> GLGDELEEVIVEKTKQTVASISSGPKHTQKVPILTANETGATMPVLPSDSIETRTTYMHFNGSETDVECFLGRAACVHVTEIQNKDAT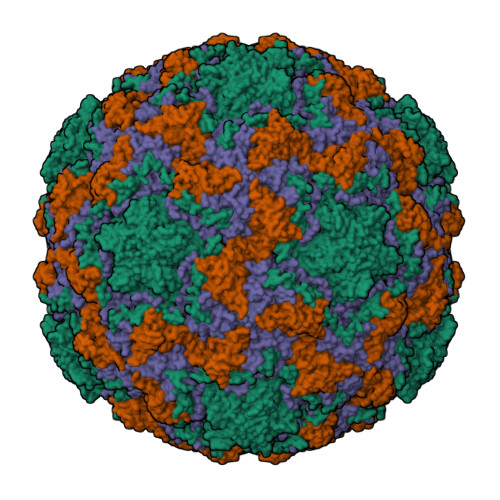GIDNHREAKLFNDWKINLSSLVQLRKKLELFTYVRFDSEYTILATASQPDSANYSSNLVVQAMYVPPGAPNPKEWDDYTWQSASNPSVFFKVGDTSRFSVPYVGLASAYNCFYDGYSHDDAETQYGITVLNHMGSMAFRIVNEHDEHKTLVKIRVYHRAKHVEAWIPRAPRALPYTSIGRTNYPKNTEPVIKKRKGDIKSY;> SPNVEACGYSDRVQQITLGNSTITTQEAANAVVCYAEWPEYLPDVDASDVNKTSKPDTSVCRFYTLDSKTWTTGSKGWCWKLPDALKDMGVFGQNMFFHSLGRSGYTVHVQCNATKFHSGCLLVVVIPEHQLASHEGGNVSVKYTFTHPGERGIDLSSAADTIGPGRAFYTTKNNEVGGPVKDVIYNMNGTLLGNLLIFPHQFINLRTNNTATIVIPYINSVPIDSMTRHNNVSLMVIPIAPLTVPTGATPSLPITVTIAPMCTEFSGIRSKSIVPQ;> GLPTTTLPGSGQFLTTDDRQSPSALPNYEPTPRIHIPGKVHNLLEIIQVDTLIPMNNTHTKDEVNSYLIPLNANRQNEQVFGTNLFIGDGVFKTTLLGEIVQYYTHWSGSLRFSLMYTGPALSSAKLILAYTPPGARGPQDRREAMLGTHVVWDIGLQSTIVMTIPWTSGVQFRYTDPDTYTSAGFLSCWYQTSLILPPETTGQVYLLSFISACPDFKLRLMKDTQTISQTVALTE;> GAQVSTQKSGSHENQNILTNGSNQTFTVINYYKDAASTSSAGQSLSMDPSKFTEPVKDLMLKGAPALN> RGSHMSLSKKRKLESGDSGGAGAGGEGAEEENGGEQ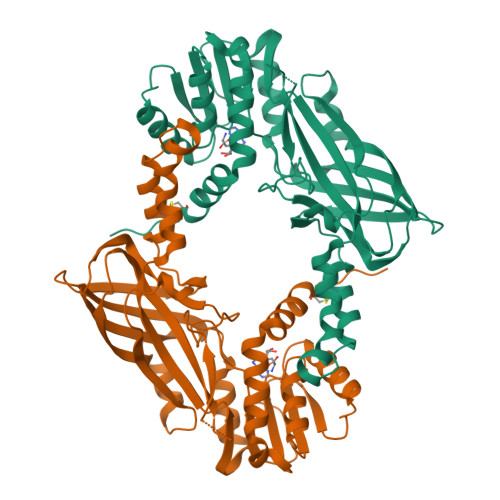EAAPPRPRRTKSERDQLYYECYSDVSVHEEMIADQVRTEAYRLGILKNWAALRGKTVLDVGAGTGILSIFCAQAGARRVYAVEASAIWQQAREVVRLNGLEDRVHVLPGPVETVELPERVDAIVSEWMGYGLLHESMLSSVLHARTKWLKEGGLLLPASAELFVAPISDQMLEWRLGFWSQVKQHYGVDMSCMESFATRCLMGHSEIVVQDLSGEDVLARPQRFAQLELARAGLEQELEAGVGGRFRCSCYGSAPLHGFAVWFQVTFPGGDSEKPLVLSTSPLHPATHWKQALLYLNEPVPVEQDTDISGEITLLPSPDNPRRLRILLRYKVGDHEEKTKDFAMED>[4x]MKAPSYHVVRGDIATATEGVIINAANSKGQPGGGVCGALYKKFPESFDLQPIEVGKARLVKGAAKHIIHAVGPNFNKVSEVEGDKQLAEAYESIAKIVNDNNYKSVAIPLLSTGIFS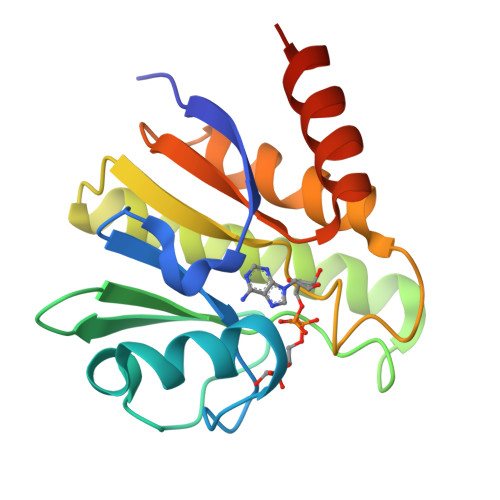GNKDRLTQSLNHLLTALDTTDADVAIYCRDKKWEMTLKEAVARREHHHHHH> MRKVKKLRLDKENTGSWRSFSLNSEGAERMATTGTPTADRGDAAATDDPAARFQVQKHSWDGLRSIIHGSRKYSGLIVNKAPHDFQFVQKTDESGPHSHRLYYLGMPYGSRENSLLYSEIPKKVRKEALLLLSWKQMLDHFQATPHHGVYSREEELLRERKRLGVFGITSYDFHSESGLFLFQ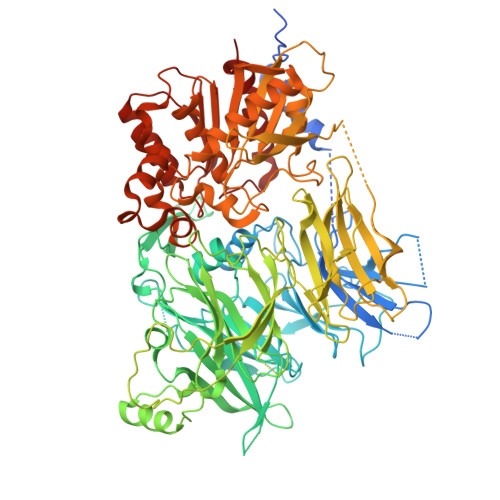ASNSLFHCRDGGKNGFMVSPMKPLEIKTQCSGPRMDPKICPADPAFFSFINNSDLWVANIETGEERRLTFCHQGLSNVLDDPKSAGVATFVIQEEFDRFTGYWWCPTASWEGSEGLKTLRILYEEVDESEVEVIHVPSPALEERKTDSYRYPRTGSKNPKIALKLAEFQTDSQGKIVSTQEKELVQPFSSLFPKVEYIARAGWTRDGKYAWAMFLDRPQQWLQLVLLPPALFIPSTENEEQRLASARAVPRNVQPYVVYEEVTNVWINVHDIFYPFPQSEGEDELCFLRANECKTGFCHLYKVTAVLKSQGYDWSEPFSPGEDEFKCPIKEEIALTSGEWEVLARHGSKIWVNEETKLVYFQGTKDTPLEHHLYVVSYEAAGEIVRLTTPGFSHSCSMSQNFDMFVSHYSSVSTPPCVHVYKLSGPDDDPLHKQPRFWASMMEAASCPPDYVPPEIFHFHTRSDVRLYGMIYKPHALQPGKKHPTVLFVYGGPQVQLVNNSFKGIKYLRLNTLASLGYAVVVIDGRGSCQRGLRFEGALKNQMGQVEIEDQVEGLQFVAEKYGFIDLSRVAIHGWSYGGFLSLMGLIHKPQVFKVAIAGAPVTVWMAYDTGYTERYMDVPENNQHGYEAGSVALHVEKLPNEPNRLLILHGFLDENVHFFHTNFLVSQLIRAGKPYQLQIYPNERHSIRCPESGEHYEVTLLHFLQEYLHHHHHH> MKTITGVFNSFDSLTWTRSVEYAYKGPETPTWNAVLGWSLNSTTADPGDTFTLILPCVFKFITTQ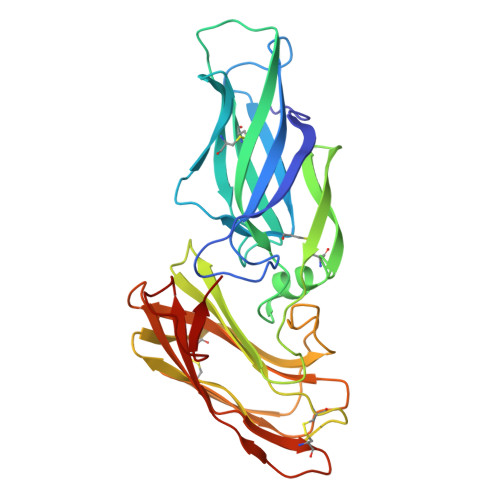TSVDLTADGVSYATCDFNAGEEFTTFSSLSCTVNSVSVSYARVSGTVKLPITFNVGGTGSSVDLADSKCFTAGKNTVTFMDGDTKISTTVDFDASPVSPSGYITSSRIIPSLNKLSSLFVVPQCENGYTSGIMGFVASNGATIDCSNVNIGISKGLNDWNFPVSSESFSYTKTCTSTSITVEFQNVPAGYRPFVDAYISAENIDKYTLTYANEYTCENGNTVVDPFTLTWWWYKNSEADSDGDVIVV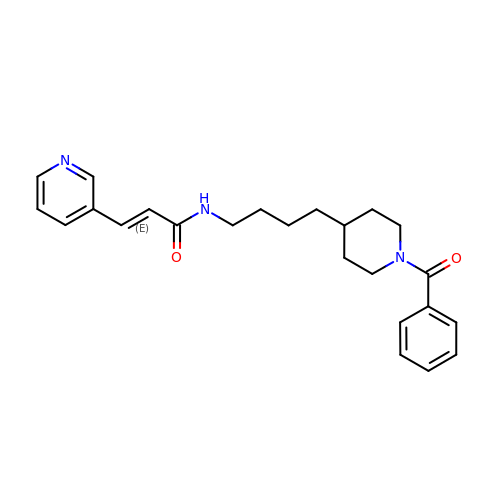(2E)-N-{4-[1-(benzenecarbonyl)piperidin-4-yl]butyl}-3-(pyridin-3-yl)prop-2-enamide | C24 H29 N3 O2 | KPBNHDGDUADAGP-VAWYXSNFSA-N N-{(1S,2R)-1-BENZYL-2-HYDROXY-3-[(3-METHOXYBENZYL)AMINO]PROPYL}-6-(ETHYLAMINO)-1-METHYL-1,3,4,5-TETRAHYDRO-2,1-BENZOTHIAZEPINE-8-CARBOXAMIDE 2,2-DIOXIDE 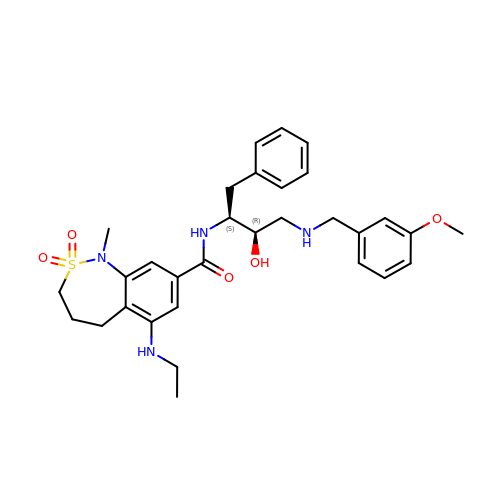| C31 H40 N4 O5 S | JAQQVYMOVUUAHB-MFMCTBQISA-N> MAIKFENVSYVYSPGSPLEAIGLDQLNFSLEEGKFIALVGHTGSGKSTLMQHFNALLKP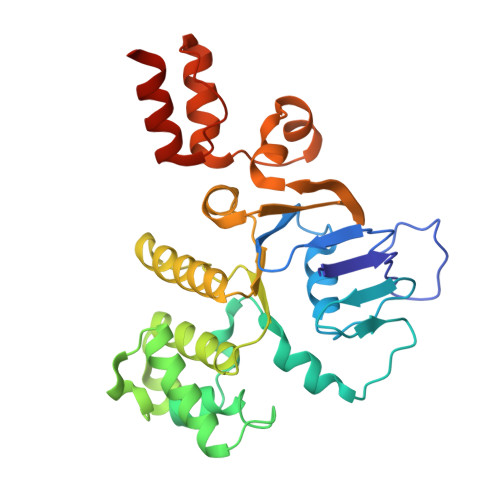TSGKIEIAGYTITPETGNKGLKDLRRKVSLAFQFSEAQLFENTVLKDVEYGPRNFGFSEDEAREAALKWLKKVGLKDDLIEHSPFDLSGGQMRRVALAGVLAYEPEIICLDEPAAGLDPMGRLEMMQLFKDYQAAGHTVILVTHNMDDVADYADDVLALEHGRLIKHASPKEVFKDSEWLQKHHLAEPRSARFAAKLEAAGLKLPGQPLTMPELADAIKQSLKGGEHE>ASMKQPVVVIGSGLAGLTTSNRLISKYRIPVVLLDKAASIGGNSIKASSGINGAHTDTQQNLKVMDTPELFLKDTLHSAKGRGVPSLMDKLTKESKSAIRWLQTEFDLKLDLLAQLGGHSVPRTHRSSGKLPPGFEIVQALSKKLKDISSKDSNLVQIMLNSEVVDIELDNQGHVTGVVYMDENGNRKIMKSHHVVFCSGGFGYSKEMLKEYSPNLIHLPTTNGKQTTGDGQKILSKLGAELIDMDQVQVHPTGFIDPNDRENNWKFLAAEALRGLGGILLHPTTGRRFTNELSTADTVTMEIQSKCPKNDNRALLVMSDKVYENYTNNINFYMSKNLIKKVSINDLIRQYD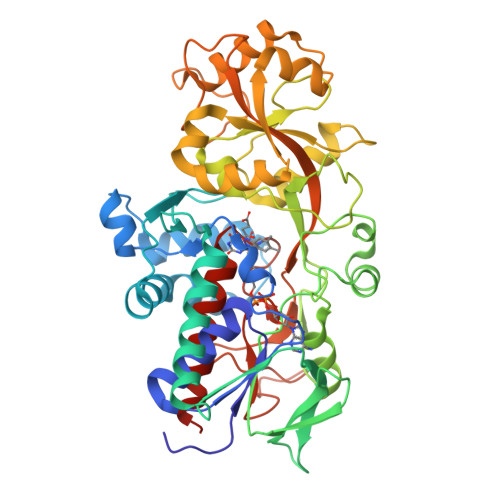LQTTASELVTELKSYSDVNTKDTFDRPLIINAFDKDISTESTVYVGEVTPVVHFTMGGVKINEKSQVIKKNSESVLSNGIFAAGEVSGGVHGANRLGGSSLLECVVFGKTAADNIAKLY[2x]TERT-BUTYL 3-[(4-OXO-3H-PYRIDO[2,3-D]PYRIMIDIN-2-YL)AMINO]AZETIDINE-1-CARBOXYLATE 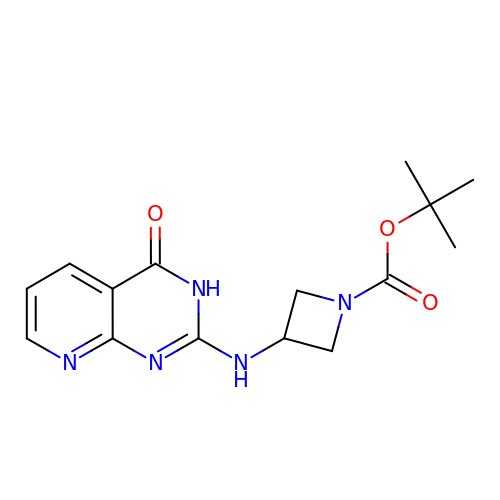| C15 H19 N5 O3 | CKUDSTVQYFRZJW-UHFFFAOYSA-N>TSVNSAEASTGAGGGGSNPVKSMWSEGATFSANSVTCTFSRQFLIPYDPEHHYKVFSPAASSCHNASGKEAKVCTISPIMGYSTPWRYLDFNALNLFFSPLEFQHLIENYGSIAPDALTVTISEIAVKDVTDKTGGGVQVTDSTTGRLCMLVDHEYKYPYVLGQGQDTLAPELPIWVYFPPQYAYLTVGDVNTQGISGDSKKLASEESAFYVLEHSSFQLLGTGGTATMSYKFPPVPPENLEGCSQHFYEMYNPLYGSRLGVPDTLGGDPKFRSLTHEDHAIQPQNFMPGPLVNSVSTKEGDSSNTGAGKALTGLSTGTSQNTRISLRPGPVSQPYHHWDTDKYVTGINAISHGQTTYGNAEDKEYQQGVGRFPNEKEQLKQLQGLNMHTYFPNKGTQQYTDQIERPLMVGSVWNRRALHYESQLWSKIPNLDDSFKTQFAALGGWGLHQPPPQIFLKILPQSGPIGGIKSMGITTLVQYAVGIMTVTMTFKLGPRKATGRWNPQPGVYPPHAAGHLPYVLYDPTATDAKQHHRHGYEKPEELWTAKSRVHPL[6x];> GLASANVDFAFSLYKQLVLKAPDKNVIFSPLSISTALAFLSLGAHNTTLTEILKGLKFNLTETSEAEIHQSFQHLLRTLNQSSDELQLS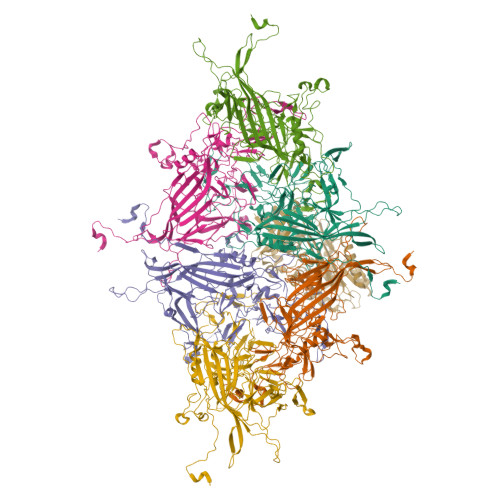MGNAMFVKEQLSLLDRFTEDAKRLYGSEAFATDFQDSAAAKKLINDYVKNGTRGKITDLIKDLDSQTMMVLVNYIFFKAKWEMPFDPQDTHQSRFYLSKKKWVMVPMMSLHHLTIPYFRDEELSCTVVELKYTGNASALFILPDQDKMEEVEAMLLPETLKRWRDSLEFREIGELYLPKFSISRDYNLNDILLQLGIEEAFTSKADLSGITGARNLAVSQVVHKAVLDVFEEGTEASAATAVKITLLSALVETRTIVRFNRPFLMIIVPTDTQNIFFMSKVTNPKQ>MASTAAETEKPEDHNDLVQLCNPHIAAMKEDILYHFSLSTSTHDFPAMFGDVKFVCVGGSPSRMKAFIKYVAMELGFAHPGADYPNICEGTDRYAMFKVGPVLSVSHGMGVPSIAIMLHELIKLLYHAHCSGVTLIRIGTSGGIGLEPGSVVITRQAVDPCFKPEFEQIVLGKREVRNTDLDEQLVQELARCSAELGEFPTVVGNTMCTLDFYEGQGRLDGALCSYTEKDKQDYLRAAYAAGIRNIEMEASVFA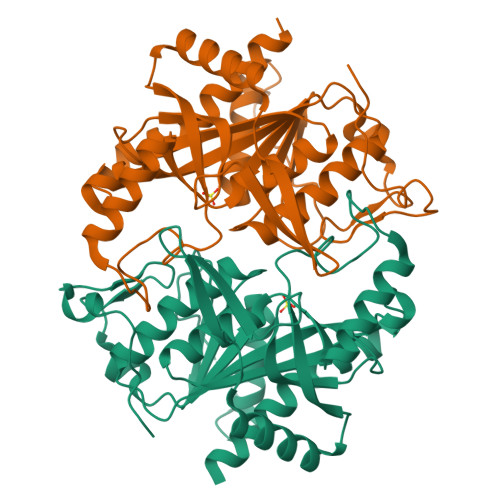AMCNACGLRAAVVCVTLLNRLEGDQISSPHDVLAEYQQRPQRLVGQFIKKRLMQA[4x]The 12-kDa FK506-binding protein (FKBP12) is a ubiquitously expressed peptidyl-prolyl isomerase with considerable homology between fungal pathogens and is thus a prime candidate for future targeting efforts to generate a panfungal strategy. PPIase proteins all catalyze the cis/trans isomerization of peptide bonds N terminal to proline residues in polypeptide chains. In addition to its role as a PPIase, FKBP12 is a member of the immunophilin family and is the target of the immunosuppressive drugs FK506 and rapamycin. Three extended loops, which have been called the 40s loop (between β2 and β3), the 50s loop (between β3′ and α1), and the 80s loop (between β4 and β5), surround a deep active-site pocket that binds both FK506 and rapamycin.

Three different crystal forms of the apo C. albicans FKBP12, to resolutions of 1.99, 2.3, and 2.4 Å, were obtained. While the C. albicans apo FKBP12 structure is very similar to previously determined FKBP12 structures, an unexpected finding that emerged from analysis of the crystal packing was that despite being obtained under very different crystallization conditions with distinct crystal lattices, all three C. albicans apo FKBP12 structures displayed the same intermolecular interactions between subunits. What is notable about this interaction is that the 80s loop of one subunit docks into the active site of the adjacent subunit and vice versa, suggesting that the loop may act as a substrate. Indeed, Pro104, which is located at the tip of the loop, is inserted most deeply into the pocket and is surrounded by residues that have been implicated, via mutagenesis, to be involved in FKBP PPIase activity. Three residues, in particular, were implicated as important for FKBP12 catalysis and correspond to Val59, Asp41, and Tyr97 in the C. albicans protein. These residues all make direct contacts with Pro104, which rests within an aromatic cleft formed by Tyr30, Phe50, and Trp63. Although most of the contacts that hold the loop in position in the active site are with the central Pro104, additional hydrophobic contacts with Ile102, Pro103, and Ile105 are provided, while Arg100 makes hydrogen bonds with the carbonyl oxygens at the edge of the pocket. Notably, the interface in the C. albicans FKBP12-FKBP12 interaction is minimal (burying 592 Å2 from solvent), which suggests that, like known substrate-enzyme complexes, the proteins form a weak interaction; typical dimer interfaces bury >2,000 Å2 of surface from solvent. Comparison of the C. albicans FKBP12 apo structure with FKBP12-FK506 structures reveals that the 80s loop binds in the same pocket as FK506. Interestingly, unlike the C. albicans apo FKBP12 structures, which were all captured with Pro104 in the cis conformation, in the A. fumigatus structure, Pro90 in one subunit was bound in the cis conformation and Pro90 in the other was bound in the trans state, thus potentially providing a snapshot of self-catalysis.

>EELPQIEIVQEGDNTTFAKPGDTVTIHYDGKLTNGKEFDSSRKRGKPFTCTVGVGQVIKGWDISLTNNYGKGGANLPKISKGTKAILTIPPNLAYGPRGIPPIIGPNETLVFEVELLGVNGQ[2x]> ELPQMTQQLNSDDMQEQLSATVKFRQILSREHRPPIDVVIQAGVVPRLVEFMRENQPEMLQLEAAWALTNIASGTSAQTKVVVDADAVPLFIQLLYTGSVEVK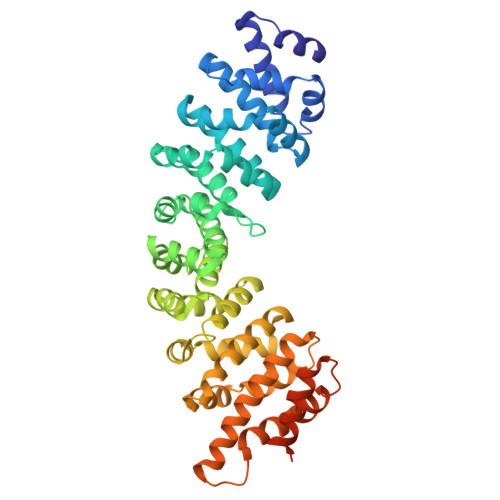EQAIWALGNVAGDSTDYRDYVLQCNAMEPILGLFNSNKPSLIRTATWTLSNLCRGKKPQPDWSVVSQALPTLAKLIYSMDTETLVDACWAISYLSDGPQEAIQAVIDVRIPKRLVELLSHESTLVQTPALRAVGNIVTGNDLQTQVVINAGVLPALRLLLSSPKENIKKEACWTISNITAGNTEQIQAVIDANLIPPLVKLLEVAEDKTKKEACWAISNASSGGLQRPDIIRYLVSQGCIKPLCDLLEIADNRIIEVTLDALENILKMGEADKEARGLNINENADFIEKAGGMEKIFNCQQNENDKIYEKAYKIIETYFGEEEDAVDETMAPQNAGNTFGFGSNVNQQFNF> SHDSLRPKLSEEQQHIIAILLDAHHKTYDPTYADFRDFRPPVRMDGSTGSVTLDLSPLSMLPHLADLVSYSIQKVIGFAKMIPGFRDLTSDDQIVLLKSSAIEVIMLRSNQSFTMDDMSWDCGSQDYKYDVTDVSKAGHTLELIEPLIKFQVGLKKLNLHEEEHVLLMAICIVSP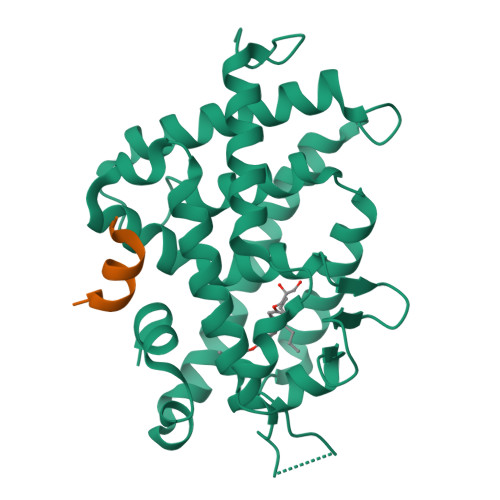DRPGVQDAKLVEAIQDRLSNTLQTYIRCRHPPPGSHQLYAKMIQKLADLRSLNEEHSKQYRSLSFQPENSMKLTPLVLEVFGN;> KNHPMLMNLLKDN>[2x]MEQSIKSKGFEHRLLLIMWGLLLSLSAFAQQITVKGHVVDATGEPVIGASVIEGKSTNGTITDIDGNFSLNVSANSALTISFVGYKTQTVSVNGKTALKVTLQEDTEVLDEVVVVGYGTMKKSDLTGAVSSVGVKDIKDSPVANIGQAMQGKVSGVQIIDAGKPGDNVTIKIRGLGTINNSNPLVVIDGIPTDLGLSSLNMADVERVDVLKDASATAIYGSRGANGVVMITSKRGAEGAGKVTVNANWAIQNATKVPDMLNAAQYAALSNDMLSNNDDNTNPYWADPSSLGKGTNWLDEMLRTGVKQSYSVSYSGGTEKAHYYVSGGFLDQSGIVKSVNYRRFNFQANSDAQVNKWLKFTTNLTFSTD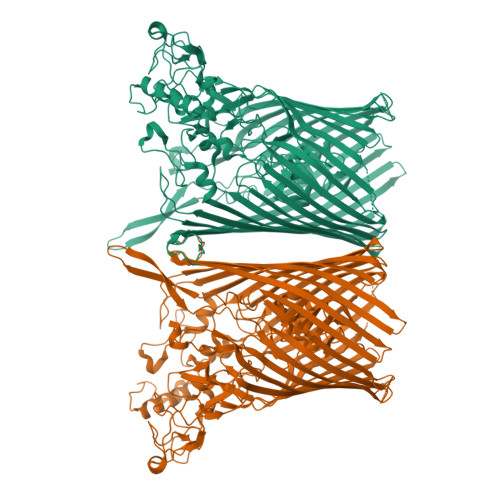VKEGGTYSIGDAMKALPTQPVKNDDGSWSGPGQEAQWYGSIRNPIGTLHMMTNETKGYNFLANITGEITFTKWLKLKSTFGYDAKFWFADNFTPAYDWKPNPVEESSRYKSDNKSFTYLWDNYFVFDHTFAKKHRVGVMAGSSAQWNNYDYLNAQKNIFMFDNIHEMDNGEKMYSLGGSQSDWALLSLMARLNYSYEDKYLLTATVRRDGSSRFGKNNRWGTFPSVSLAWRVSQEDWFPKDNFLMNDLKLRVGYGVTGNQEIGNYGFVASYNTGVYPFGNNNSTALVSTTLSNPNIHWEEVRQANFGVDMSLFDSRVSLSLDAYIKNTNDMLVKASIPITSGFEDTTETFTNAGKMRNKGVEMTLRTINLKGIFSWESALTATYNKNEILDLNSETPMFINQIGNSYVTMLKAGYPINVFYGYVTDGLFQNWGEVNRHATQPGAAPGDIRFRDLNNDGVINDEDRTILGNPNPNWFFSLSNNLSYKGWELSVFLQGVAGNKIYNANNVDNEGMAAAYNQTTAVLNRWTGEGTSYSMPRAIWGDPNQNCRVSDRFVENGSYLRLKNITLSYTLPKKWLQKIQLENARISFSCENVATITRYSGFDPEVDVNGIDSSRYPISRTFSMGLNFNF> MDEFEMIKRNTSEIISEEELREVLKKDEKSALIGFEPSGKIHLGHYLQIKKMIDLQNAGFDIIILLADLHAYLNQKGELD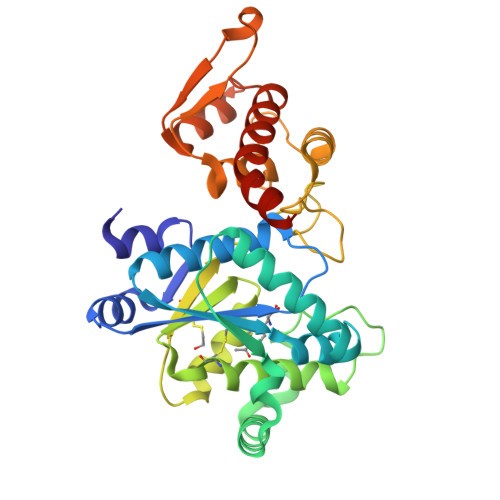EIRKIGDYNKKVFEAMGLKAKYVYGSEFQLDKDYTLNVYRLALKTTLKRARRSMELIAREDENPKVAEVIYPIMQVNGCHYRGVDVAVGGMEQRKIHMLARELLPKKVVCIHNPVLTGLDGEGKMSSSKGNFIAVDDSPEEIRAKIKKAYCPAGVVEGNPIMEIAKYFLEYPLTIKRPEKFGGDLTVNSYEELESLFKNKELHPMDLKNAVAEELIKILEPIRKRLLEHHHHHH>[4x]MSYTVGTYLAERLVQIGLKHHFAVAGDYNLVLLDNLLLNKNMEQVYCCNELNCGFSAEGYARAKGAAAAVVTYSVGALSAFDAIGGAYAENLPVILISGAPNNNDHAAGHVLHHALGKTDYHYQLEMAKNITAAAEAIYTPEEAPAKIDHVIKTALREKKPVYLEIACNIASMPCAAPGPASALFNDEASDEASLNAAVDETLKFIANRDKVAVLVGSKLRAAGAEEAAVKFTDALGGAVATMAAAKSFFPEENALYIGTSWGEVSYPGVEKTMKEADAVIALAPVFNDYSTTGWTDIPDPKKLVLAEPRSVVVNGIRFPSVHLKDYLTRLAQKVSKKTGSLDFFKSLNAGELKKAAPADPSAPLVNAEIARQVEALLTPNTTVIAETGDSWFNAQRMKLPNGARVEYEMQWGHIGWSVPAAFGYAVGAPERRNILMVGDGSFQ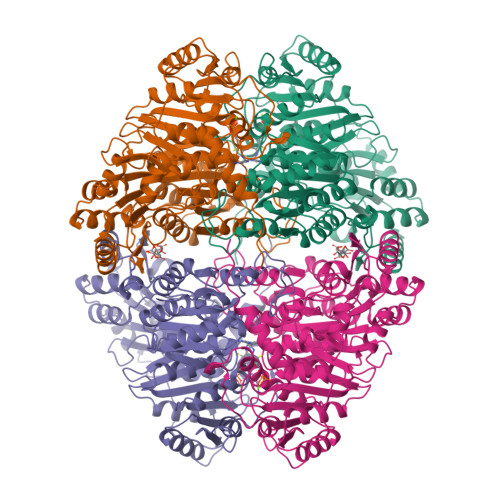LTAQEVAQMVRLKLPVIIFLINNYGYTIEVMIHDGPYNNIKNWDYAGLMEVFNGNGGYDSGAAKGLKAKTGGELAEAIKVALANTDGPTLIECFIGREDCTEELVKWGKRVAAANSRKPVNKVV> MAVTDLSLTNSSLMPTLNPMIQQLALAIAASWQSLPLKPYQLPEDLGYVEGRLEGEKLVIENRCYQTPQFRKMHLELAKVGKGLDDLHCVMFPEPLYGLPLFGCDIVAGPGGVSAAIADLSPTQSDRQLPAAYQKSLAELGQPEFEQQRELPPWGEIFSEYCL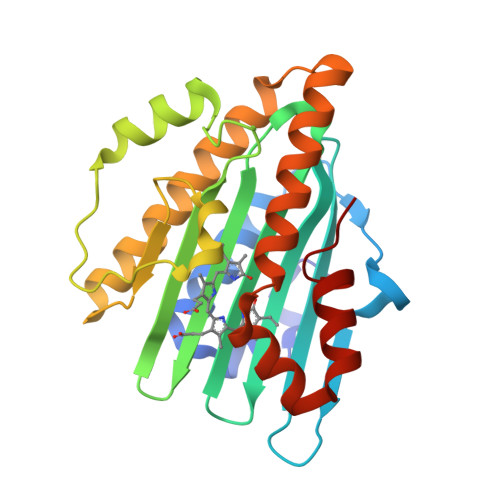FIRPSNVTEEERFVQRVVDFLQIHCHQSIVAEPLSEAQTLEHRQGQIHYCQQQQKNDKTRRVLEKAFGEAWAERYMSQVLFDVIQ> MQNIVSSKSEQATVIGLVGFYFKDSTFKELMFIQVGEKSNLMNKARINTDAQQIQSIRWMGNLKSPQTGEYRLSTSSDENVILQINGETVINQASIQKNLKLEANQVYEIKIEYRNTSNTLPDLQLFWSMNNAQKEQIPEKYILSPNFSEKANSLAEKETQSFFPNYNLFDRQQENGEKQSMSTPVDTDNDCIPDEWEEKGYTFRNQQIVPWNDAYSAEGYKKYVSNPYHARTVKDPYTDFEKVTGHMPAATKYEARDPLVAAYPSVGVGMEKLHFSKNDTVTEGNADTKSKTTTKTDTTTNTVEIGGSLGFSDKGFSFSISPKYTHSWSSSTSVADTDSTTWSSQIGINTAERAYLNANVRYYNGGTAPIYDLKPTTNFVFQNSGDSITTITAGPNQIGNSLGAGDTYPQKGQAPISLDKANEAGTVKIAINAEQLDKIQAGTEILNIETTQNRGQYGILDEKGQVIPGGEWDPIRTNIDAVSGSLTLNLGTGKDSLERRVAAKNMNDPEDKTPEITIKEAIKKAFNAYYYDGRLYYTDQGEKDIFIDEPSINLITDENTKKEIERQLNQMPGKTVYDVKWKRGMKITLHVPIKYYDFETSENLWYYTYQESGGYTGKKRGRIGTDGHGTAMSNPQLKPYTSYTVRAYVRTASTTGSNEVVFYADNSSGNGQGAKVSGKVTGGKWKIAEFSFNTFNNPEYFKIIGLKNNGNANLHFDDVSVIEWKTNENLQKKHIFEKWSFGSNDEMVIGATFTRVPSSKIRYQWKINGRLGSIIPAPPLDANGKRTVTYGSITAITPMELYAVDEKNDNLKVKVAELGESEIEKVMIDAHKFSGWWYLSENPNLYSGLSLYKLPDIFYNNVSSYKIRVNGKKVQTVSKPSPFLFQITFNLKNPNGGTYPTKDASVELWATVGGKDLKVLHKWIQKSDVMYSQTNN

In the current study we determined the crystal structure and mode of action (MOA) of the Vpb4Da2 protein (formerly known as Vip4Da2) from Bt, the first identified insecticidal Vpb4 protein with commercial level control against WCR. Amino acid sequence analysis designates Vpb4Da2 as a new β-PFP member of the Bacterial_exotoxin_B protein family (IPR035088) with Vpb4Da2 domain architecture composed of PA14 (PF07691) and Binary-toxB (PF03495) protein family (Pfam) domains. The Vpb4Da2 structure exhibits a six-domain architecture mainly comprised of antiparallel β-sheets organized into β-sandwich layers. Functional assessment of Vpb4Da2 suggests that domains 4–6 comprise the WCR receptor binding region and are key in conferring the observed insecticidal activity against WCR.

The structure of Vpb4Da2 was solved by X-ray crystallography to 3.2 Å resolution in the space group C2221 with one molecule in the asymmetric unit. Domain 1 (amino acids 1–263), which encompasses a characteristic PA14 domain, adopts a conformation of ten anti-parallel β-strands, six small α-helices, and binds two adjacent calcium ions visible in the structure. Domain 2 (amino acids 264–483) consists of a β-hairpin motif, seven anti-parallel β-strands, a partially structured long loop, and three additional α-helices. Domain 4 (amino acids 594–730) consists of β-strands exhibiting a classical β-jelly roll fold and harboring a calcium ion. Domain 5 (amino acids 731–820) has an immunoglobulin-like fold of six β-strands and one α-helix. Domain 6 (amino acids 821–937), like domain 5, adopts an immunoglobulin-like fold with seven β-strands and two α-helices. Vpb4Da2 exhibits an overall β-strand-rich structure and shares structural homology to PA, namely the domain conformation and organization spanning approximately the first 600 amino acids that include domains 1–3. Furthermore, unlike the PA domain 4 described as a receptor binding domain with an immunoglobulin-like fold, Vpb4Da2 domain 4 adopts a fold of the carbohydrate binding module 6 (CBM6), which is also found in domain 3 of many three-domain Cry proteins. Another key aspect of Vpb4Da2’s unique domain 5 and 6 C-terminal extension is that they connect to domain 4 at a structurally identical position where PA has its receptor binding epitope. Given this steric occlusion, the Vpb4Da2 structure suggests that it has a different receptor recognition site than PA, likely comprised by its domains 5 and 6 or domains 4 through 6.>[4x]QDNCTCPTNKMTVCSPDGPGGRCQCRALGSGMAVDCSTLTSKCLLLKARMSAPKNARTLVRPSEHALVDNDGLYDPDCDPEGRFKARQCQQTSVCWCVNSVGVRRTDKGDLSLRCDELVRTHHILIDLRHRPTAGAFNHSDLDAELRRLFRERYRLHPKFVAAVHYEQPTIQIELRQQTSQKAAGDVDIGDAAYYFERDIKGESLFQGRGGLDLRVRGEPLQVERTLIYYLDEIPPKFSMKRLTHHHHHH

Trop2 (trophoblast cell surface antigen 2) is cell-surface transmembrane type-1 glycoprotein expressed in normal epithelial cells of various tissues. Trop2 and EpCAM are, in terms of amino acid sequence identity, very similar (48%). They are composed of three topological regions: ectodomain representing the largest portion of the protein, a single transmembrane region, and a short cytosolic tail. Analogous proteolytic cleavages were also demonstrated for Trop2 where cleavage at the α-site by TACE (also known as a disintegrin and metalloproteinase (ADAM) 17) within the ectodomain is followed by intramembrane cleavage by the γ-secretase complex.

For crystallization a mutant variant of Trop2 ectodomain was used where two putative N-glycosylation sites were mutated (N120Q, N208Q) while the two other sites were left intact (N33, N168) to achieve adequate balance between protein sample homogeneity and solubility. Four copies of Trop2 ectodomain were located within the asymmetric unit (chains A to D) which form various assemblies as discussed in the next section. Domains ND (Q31–L69), TY (T70–L148) and CD (V149–T274) form a triangular arrangement where each domain forms contacts with the other two. The fold of the ND and TY is stabilized by three disulfide bridges with the same cysteine–cysteine connectivity as observed in EpCAM. Interestingly, the TY-loop adopts two distinct conformations: one in chains A and B, and the other in chains C and D. Electron density corresponding to the attached carbohydrate moiety was identified only at N168 and modelled as N-acetylglucosamine (NAG) in chains C and D, and as a short branched NAG-[a-(1-6)-FUC]-NAG in chains A and B (GlycoCT notation, FUC stands for fucose). Of these five assemblies, only assembly 1 has a very large interface area of 2474 Å2 (average of interfaces between AD and BC). A large portion of the dimer interface is formed between TY-loop of one subunit and the concave β-sheet of the juxtaposed CD (βCD). The angle defined by the β-sheet and the dimer interface plain is in Trop2 very narrow (10°) and the ND is almost colinear with the plain. As noted, in EpCAM dimer dissociation/destabilization is needed to reveal the α-site, while in the tighter Trop2 dimer the α-site is accessible even in the dimeric form.2,6-DIFORMYL-4-METHYLPHENYL DIHYDROGEN PHOSPHATE | C9 H9 O6 P | 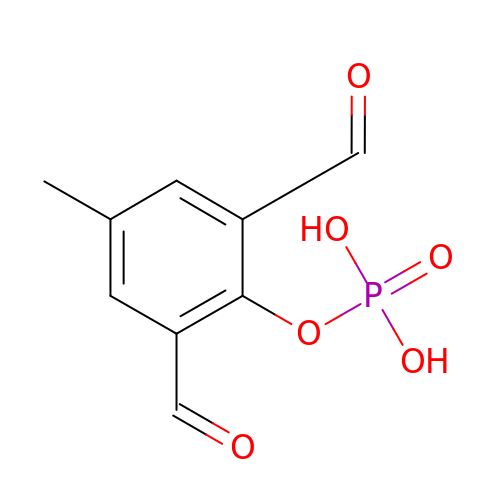NAYNUXXSJZLKPW-UHFFFAOYSA-N> GGCCAGAUCUGAGCG;> GCUCUCUGGC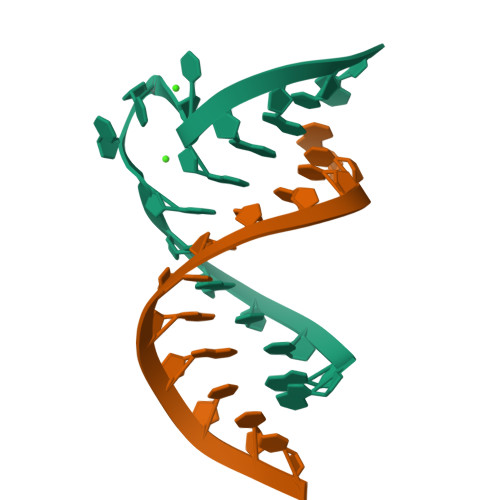CC> GPQSSKRSSRSVEDDKEGHLVCRIGDWLQERYEIVGNLGEGTFGKVVECLDHARGKSQVALKIIRNVGKYREAARLEINVLKKIKEKDKENKFLCVLMSDWFNFHGHMCIAFELLGKNTFEFLKENNFQPYPLPHVRHMAYQL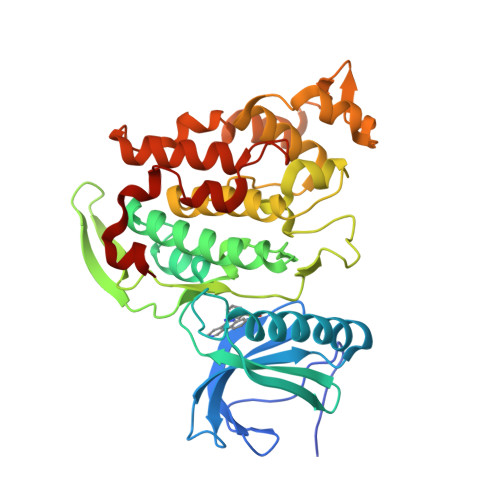CHALRFLHENQLTHTDLKPENILFVNSEFETLYNEHKSCEEKSVKNTSIRVADFGSATFDHEHHTTIVATRHYRPPEVILELGWAQPCDVWSIGCILFEYYRGFTLFQTHENREHLVMMEKILGPIPSHMIHRTRKQKYFYKGGLVWDENSSDGRYVKENCKPLKSYMLQDSLEHVQLFDLMRRMLEFDPAQRITLAEALLHPFFAGLTPEERSFHT> SDELYRQSLEIISRYLREQATGAKDTKPMGRSGATSRKALETLRRVGDGVQRNHETAFQGMLRKLDIKNEDDVKSLSRVMIHVFSDGVTNWGRIVTLISFGAFVAKHLKTINQESCIEPLAESITDVLVRTKRDWLVKQRGWDGFVEFFHVE;> PPEIAWLADAVGLKDA

Here we introduce RFpeptides, a denoising diffusion-based pipeline for designing macrocyclic binders against protein targets of interest. We tested 20 or fewer designed macrocycles against each of four diverse proteins and obtained binders with medium to high affinity against all targets. X-ray structures for macrocycle-bound myeloid cell leukemia 1, γ-aminobutyric acid type A receptor-associated protein and RbtA complexes match closely with the computational models, with a Cα root-mean-square deviation < 1.5 Å to the design models. RFpeptides is not limited to generating macrocycles with particular motifs or topologies; the diffusion process generates macrocycles with diverse shapes and sizes and selects the topologies appropriate for the protein being targeted. Among the four targets tested here, binders for MCL1 and MDM2 have helical motifs, binders for GABARAP have a β-sheet topology and binders for RbtA sample looplike conformations that make extensive contacts with the flat surface of this target.

MCL1 is also a promising target for anticancer therapeutics because of its roles in autophagy, cell survival, DNA repair and cellular proliferation. Despite specifying no hotspots to guide the generation process to a specific patch on the MCL1 structure, all selected designs bound to the functionally relevant MCL1–BH3 interaction site. Three macrocycles showed binding to the MCL1, with the best binder, MCB_D2 (MCL1 binding design 2), demonstrating a binding affinity of 2 µM. To confirm whether the designed macrocycle adopts the designed structure and engages MCL1 in the designed binding mode, we determined the X-ray crystal structure of MCB_D2 bound to MCL1 at 2.1 Å resolution. The crystal structure was nearly identical to the design model, with a root-mean-square deviation (r.m.s.d.) of 0.7 Å over all of the Cα atoms of the macrocycle with target chains aligned and Cα r.m.s.d. of 0.4 Å within the macrocycles when aligned. The side-chain rotamers of the interacting residues in the crystal structure also closely matched the design model. The crystal structure also confirmed that the binding interactions are not restricted to the helix region of the designed macrocycle but are also contributed by the loop regions. While several hydrophobic interactions from the MCB_D2 helical segment are similar to those seen in natural MCL1 binders (for example, BH3 peptide),, the N-to-C orientation of the helix is flipped in the case of MCB_D2. The loop region of MCB_D2 makes additional hydrophobic contacts and a cation–π interaction with MCL1 that we did not observe in previously reported natural MCL1 binders and their analogs. All three hits with an observable binding signal at 100 µM featured this cation–π interaction.> GSHMRNELEEMQRRADQLADESLESTRRMLQLVEESKDAGIRTLVMLDEQGEQLDRVEEGMNHINQDMKE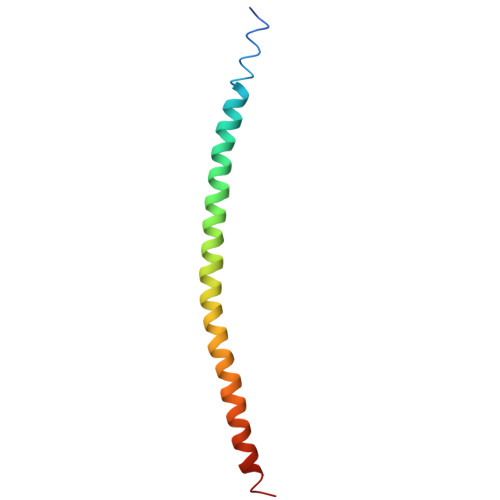AEKNLKDLGK>[4x]MKVLVTGFEPFGGEKINPTERIAKDLDGIKIGDAQVFGRVLPVVFGKAKEVLEKTLEEIKPDIAIHVGLAPGRSAISIERIAVNAIDARIPDNEGKKIEDEPIVPGAPT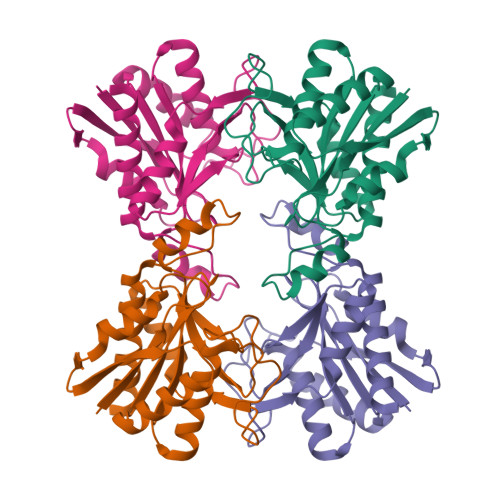AYFSTLPIKKIMKKLHERGIPAYISNSAGLYLSNYVMYLSLHHSATKGYPKMSGFIHVPYIPEQIIDKIGKGQVPPSMSYEMDLEAVKVAIEVALEELL4-[1-(2-fluorophenyl)-1H-pyrazol-4-yl]-3-[(piperidin-4-yl)methoxy]pyridine | C20 H21 F N4 O | 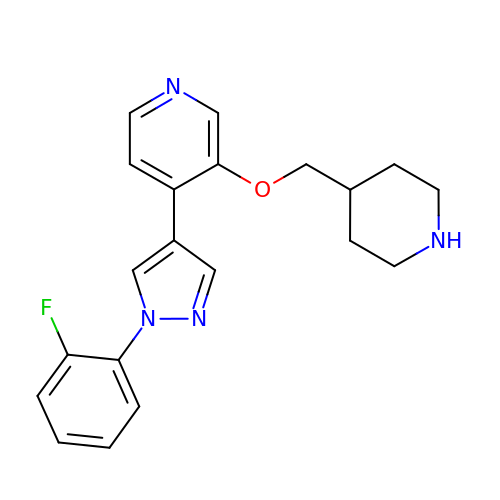GZSRUYQFWHDLJI-UHFFFAOYSA-N>[2x]MAEIPKEMLRAQTNVILLNVLKQGDNYV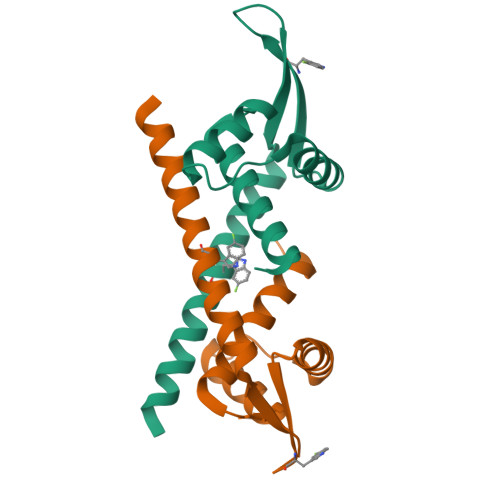YGIIKQVKEASNGEMELNEATLYTIFKRLEKDGIISSYWGDESQGGRRKYYRLTEIGHENMRLAFESWSRVDKIIENLEANKKSEAIKHHHHHH>GPSKIEEVKSTTKTQRIASHSHVKGLGLDESGLAKQAASGLVGQENAREACGVIVELIKSKKMAGRAVLLAGPPGTGKTALALAIAQELGSKVPFCPMVGSEVYSTEIKKTEVLMENFRRAIGLRIKEGPPGIIQDVTLHDLDVANARPQGGQDILSMMGQLMKPKKTEITDKLRGEINKVVNKYIDQGIAELVPGVLFVDEVHMLDIECFTYLHRALESSIAPIVIFASNRGNCVIRGTEDITSPHGIPLDLLDRVMIIRTMLYTPQEMKQIIKIRAQTEGINISEEALNHLGEIGTKTTLRYSVQLLTPANLLAKINGKDSIEKEHVEEISELFYDAKSSAKILADQQDKYMK[6x];>[6x]GGSMATVTATTKVPEIRDVTRIERIGAHSHIRGLGLDDALEPRQASQGMVGQLAARRAAGVVLEMIREGKIAGRAVLIAGQPGTGKTAIAMGMAQALGPDTPFTAIAGSEIFSLEMSKTEALTQAFRRSIGVRIKEGPPGVVHTVSLHEIDVINSRTQGFLALFSGDTGEIKSEVREQINAKVAEWREEGKAEIIPGVLFIDEVHMLDIESFSFLNRALESDMAPVLIMATNRGITRIRGTSYQSPHGIPIDLLDRLLIVSTTPYSEKDTKQILRIRCEEEDVEMSEDAYTVLTRIGLETSLRYAIQLITAASLVCRKRKGTEVQVDDIKRVYSLFLDESRSTQYMKEYQDAF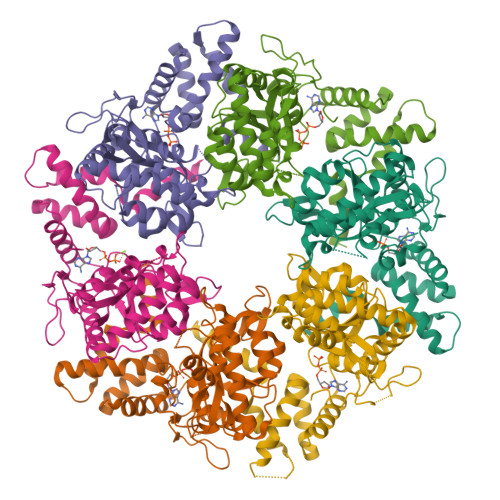LFNELKGETMDTS> ASVCFVKALYDYEGQTDDELSFPEGAIIRILNKENQDDDGFW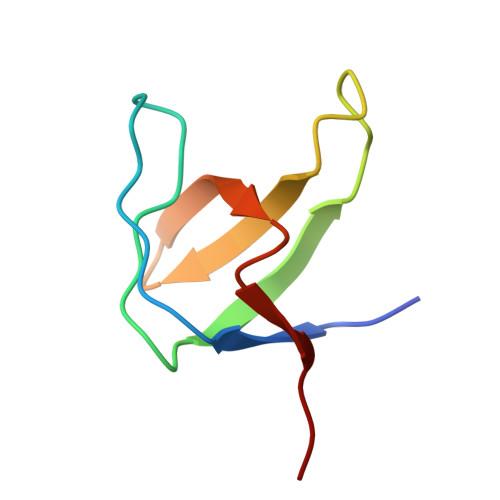EGEFNGRIGVFPSVLVEELSA GP is an allosteric enzyme that catalyses the first step of glycogen degradation in the liver and muscle to produce glucose-1-phosphate. GP senses plasma levels of glucose to ensure that glycogenolysis is halted when glucose is abundant in plasma. This is achieved through allosteric binding of glucose to GP and stabilization of a conformation that enables the inactivation of the enzyme. Here, we present the structure-based design and organic synthesis of two new GP glucopyranosyl inhibitors as well as the kinetic and X-ray crystallography assessment of the new compounds.

Within the series of tested molecules, 4 proved to be the most potent inhibitor with a Ki of 9.7 μM against rmGPb and 19.4 μM against the pharmacologically relevant hlGPa. However, the two compounds bind significantly different at the enzyme active site and the biphenyl moieties point to different directions as a result of their meta and para connection, respectively. Instead, in the 4 complex, atom O2 of the linker forms a hydrogen bond to the main chain amide of Leu136, a hydrogen bond previously observed for other acyl-glucopyranose derivative complexes. Structural comparison of the rmGPb-4 complex with the rmGPb-2 complex reveals that although the glucopyranose atoms are at almost identical positions at the active site C1′ shifts by ~0.4 Å to best orient the biphenyl moiety (there is a 47° inclination between the phenyl rings of 2 and 4) and hence the hydrogen bond of N1 to the main chain carbonyl oxygen of His377 is lost (distance in the rmGPb-4 complex, 4.2 Å). However, this loss is compensated by the formation of a hydrogen bond of O2 to the main chain amide of Leu136. Therefore, it seems that the 15 additional van der Waals contacts (applying a distance cut off of 4.0 Å using the program CONTACT as implemented in CCP4) of the terminal phenyl group with the protein residues at the active site are the reason for the 8.3 times lower Ki value of 4 with respect to that of 2. Furthermore, despite the fact that the two terminal phenyl groups of 3 and 4 are inclined by ~15° to each other, both are involved in cation-π stacking interactions to the imidazole ring of His341. Thus, the structural basis of the variation in the inhibitory potency between 3 and 4 seems to lie within the energy cost associated with the significant conformational change of the 280s loop triggered by the binding of 3 but not by the binding of 4. For compound 4 the congruence is even more striking as the docked pose and the observed orientation in the co-crystal structure are identical.

> MSRPLSDQEKRKQISVRGLAGVENVTELKKNFNRHLHFTLVKDRNVATPRDYYFALAHTVRDHLVGRWIRTQQHYYEKDPKRIYYLSLEFYMGRTLQNTMVNLALENACDEATYQLGLDMEELEEIEEDAGLGNGGLGRLAACFLDSMATLGLAAYGYGIRYEFGIFNQKICGGWQMEEADDWLRYGNPWEKARPEFTLPVHFYGRVEHTSQGAKWVDTQVVLAMPYDTPVPGYRNNVVNTMRLWSAKAPNDFNLKDFNVGGYIQAVLDRNLAENISRVLYPNDNFFEGKELRLKQEYFVVAATLQDIIRRFKSSKFGCRDPVRTNFDAFPDKVAIQLNDTHPSLAIPELMRVLVDLERLDWDKAWEVTVKTCAYTNHTVLPEALERWPVHLLETLLPRHLQIIYEINQRFLNRVAAAFPGDVDRLRRMSLVEEGAVKRINMAHLCIAGSHAVNGVARIHSEILKKTIFKDFYELEPHKFQNKTNGITPRRWLVLCNPGLAEIIAERIGEEYISDLDQLRKLLSYVDDEAFIRDVAKVKQENKLKFAAYLEREYKVHINPNSLFDVQVKRIHEYKRQLLNCLHVITLYNRIKKEPNKFVVPRTVMIGGKAAPGYHMAKMIIKLITAIGDVVNHDPVVGDRLRVIFLENYRVSLAEKVIPAADLSEQISTAGTEASGTGNMKFMLNGALTIGTMDGANVEMAEEAGEENFFIFGMRVEDVDRLDQRGYNAQEYYDRIPELRQIIEQLSSGFFSPKQPDLFKDIVNMLMHHDRFKVFADYEEYVKCQERVSALYKNPREWTRMVIRNIATSGKFSSDRTIAQYAREIWGVEPSRQRLPAPDEKIP(2S)-3-(4-cyanophenoxy)-N-[4-cyano-3-(trifluoromethyl)phenyl]-2-hydroxy-2-methylpropanamide | C19 H14 F3 N3 O3 | 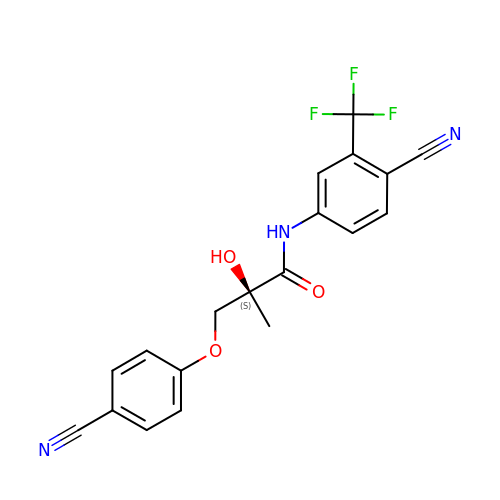JNGVJMBLXIUVRD-SFHVURJKSA-N>[2x]MPATHHSSATSAERPTVVGRIPVLDVRPVVQRGRRPAKAVTGESFEVSATVFREGHDAVGANVVLRDPRGRPGPWTPMRELAPGTDRWGATV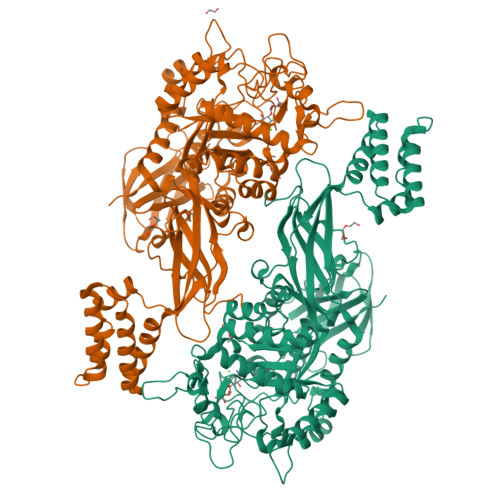TAGETGTWSYTVEAWGDPVTTWRHHARIKIPAGLDTDLVLEEGARLYERAAADVPGREDRRELLAAVDALRDESRPAASRLAAALTPQVDAVLARHPLRDLVTSSDPLPLLVERERALYGAWYEFFPRSEGTPHTPHGTFRTAARRLPAIAAMGFDVVYLPPIHPIGTTHRKGRNNTLSATGDDVGSPWAIGSPEGGHDSIHPALGTLDDFDHFVTEAGKLGLEIALDFALQCSPDHPWVHKHPEWFHHRPDGTIAHAENPPKKYQDIYPIAFDADPDGLATETVRILRHWMDHGVRIFRVDNPHTKPVAFWERVIADINGTDPDVIFLAEAFTRPAMMATLAQIGFQQSYTYFTWRNTKQELTEYLTELSGEAASYMRPNFFANTPDILHAYLQHGGRPAFEVRAVLAATLSPTWGIYSGYELCENTPLREGSEEYLDSEKYQLKPRDWTRAAREGTTIAPLVTRLNTIRRENPALRQLRDLHFHPTDKEEVIAYSKRQGSNTVLVVVNLDPRHTQEATVSLDMPQLGLDWHESVPVRDELTGETYHWGRANYVRLEPGRTPAHVCTVLRPSHPQIGGSHTTALHHHHHH>GSGGGMFGAFVSHRLWSDSGCTTTCITNSIANYVAFGEQIGFPFKSAQVFIAGPRKAVINIQEDDKVELLKMIVKHNLWVVAHGTYLDVPWSRRSAFVTHFIQQELLICKEVGIKGLV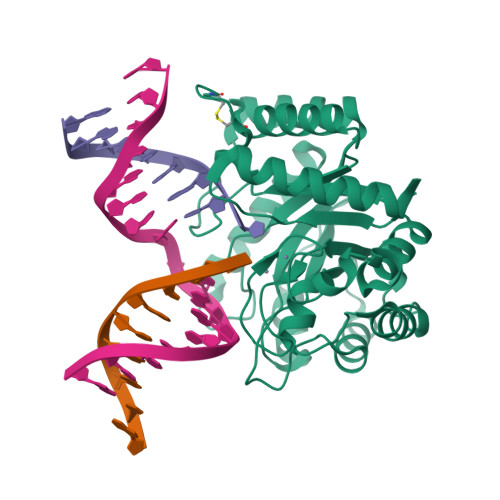LHLGAVEPELIVEGLKKIKPVEGVVIYLETPHNKHHTYKYSTMEQIKELFLRIRNTRLKQIGLCIDTAHIWSSGVNISSYNDAGQWLRSLENIHSVIPPSHIMFHLNDAATECGSGIDRHASLFEGMIWKSYSHKIKQSGLYCFVEYITRHQCPAILERNLGSSMQLQTALTAEFTTLKSLLK[2x]> TQQLFNTTT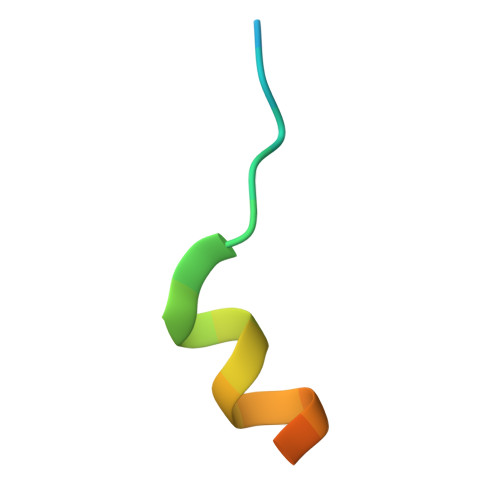MDDVYNYIFDNDE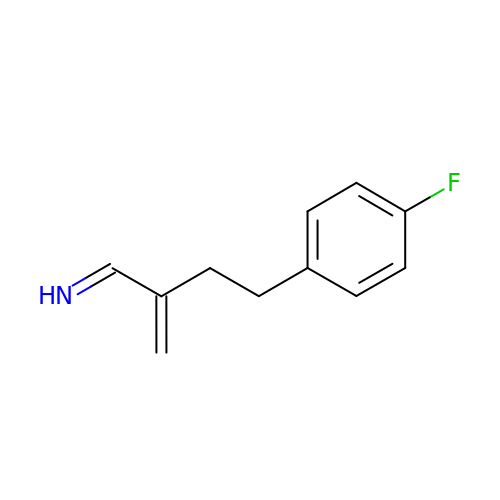(1Z)-4-(4-FLUOROPHENYL)-2-METHYLIDENEBUTAN-1-IMINE | C11 H12 F N | CFVUPEQWSFCCFT-MDWZMJQESA-N> SSSHPIFHRGEFSVCDSVSVWVGDKTTATDIKGKEVMVLGEVNINNSVFKQYFFETKCRDPNPVDSGCRGIDSKHWNSYCTTTHTFV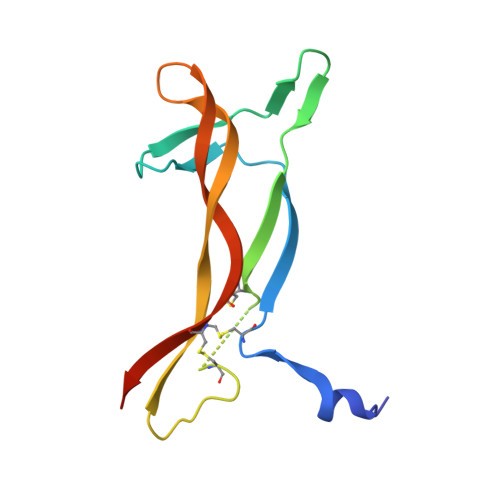KALTMDGKQAAWRFIRIDTACVCVLSRKAVRRA>[4x]MPMRKRFGQHFLHDSFVLQKIVSAIHPQ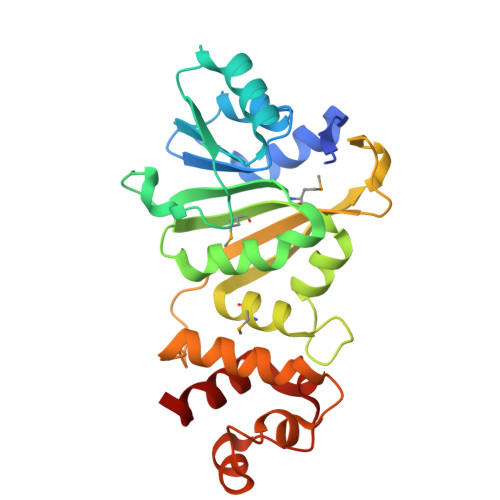KTDTLVEIGPGRGALTDYLLTECDNLALVEIDRDLVAFLQKKYNQQKNITIYQNDALQFDFSSVKTDKPLRVVGNLPYNISTPLLFHLFSQIHCIEDMHFMLQKEVVRRITAEVGSHDYGRLSVMAQYFCDNTYLFTVSPQAFTPPPRVESAIIRLIPRHNFTPVAKNLDQLSHVVKEAFSYRRKTVGNALKKLINPSQWPLLEINPQLRPQELTVEDFVKISNILN> MVFHYTNFVQETNAWWLRRVRPVYCTVLAYYGWWLYDRYYLFGKNATQDI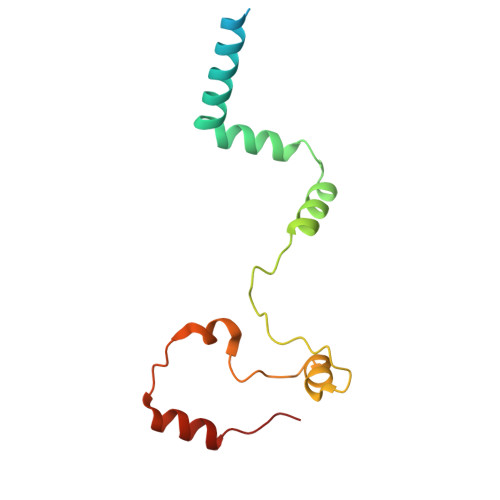RKDTTEVWEKRAALNKRNWGYNAHYKPELERSMKKVLYADPNYKFPIEWPERYMAETKTLEQVMDEEENWEYYK> GHMAKTYDYLFKLLLIGDSGVGKTCVLFRFSEDAFNSTFISTIGIDFKIRTIELDGKRIKLQIWDTAGQERFRTITTAYYRGAMGIMLVYDITNEKSFDNIRNWIRNIEEHASADVEKM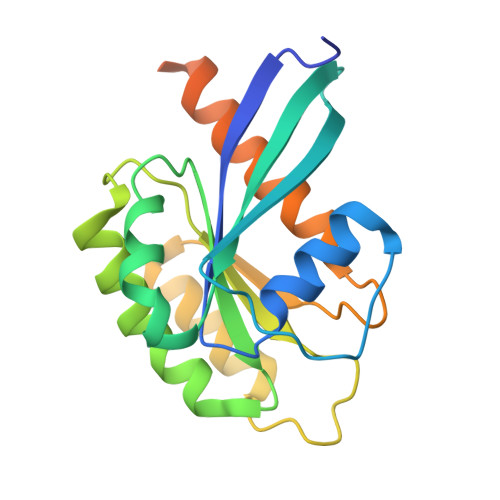ILGNKCDVNDKRQVSKERGEKLALDYGIKFMETSAKANINVENAFFTLARDIKAKMDKKLEGNSPQGSNQGVKITPDQQKRSSFFRCVLL> MSILISPDNNTGWGLHSAGMYGGAKRRSSQHPVRVRGHYRAPWGAHTRGIISGRTTVDDVIDSVVADARRYQRPTSTVDSVIDSVVADARRYAQRKSRLRRRRRRP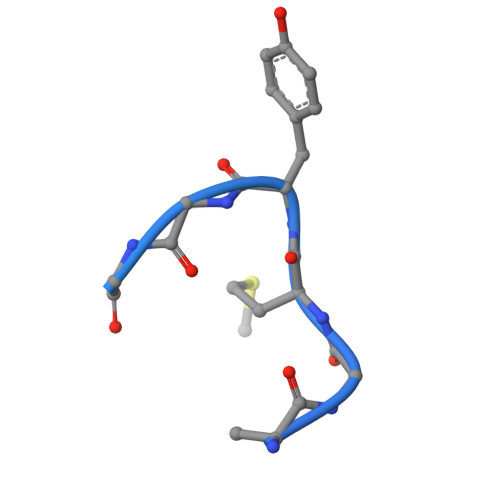TTAMIAARAVLRRARRIGRRAMRRAAAAASAGRARRQAARQAAAAIASMAQPRRGNVYWVRDASGVRVPVRTRPPRS>GSHMSQSLFSLAFGVGTQNRQEAWLEVFYALPLLKPSSEIVAAVAPILGYAAGNQALTFTSQQAYQLADALKGIDAAQSALLSRLAESQKPLVATLLAEDAAPSSTAEAYLKLHLLSHRLVKPHAVNLSGIFPLLPNVAWTNIGAVDLAELAELQLEARLKGKLLEVFSVDKFPKMTDYVVPAGVRIADTARVRLGAYIGEGTTVMHEGFVNFNAGTEGPGMIEGRVSAGVFVGKGSDLGGGCSTMGTLSGGGNIVISVGEGCLIGANAGIGIPLGDRNIVEAGLYITAGTKVALLDEQNALVKVVKARDLAGQPDLLFRRNSQNGAVECKTN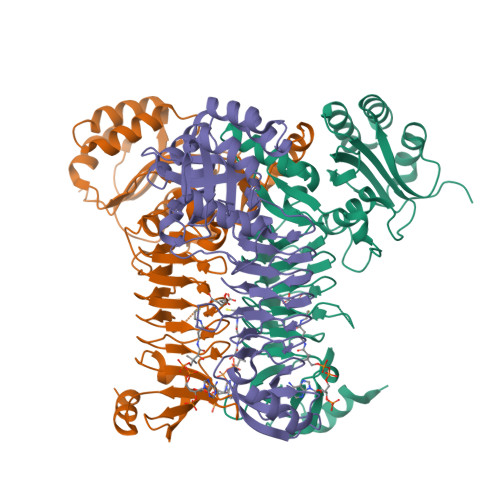KTAIELNEALHAHN[3x]>MSIQHFRVALIPFFAAFCLPVFAHPETLVKVKDAEDKLGARVGYIELDLNSGKILESFRPEERFPMMSTFKVLLCGAVLSRVDAGQEQLGRRIHYSQNDLVEYSPVTEKHLTDGMTVRELCSAAITMSDNTAANLLLTTIGGPKELTAFLHNMGDHVTRLDRWEPELNEAIPNDERDTTTPAAMATTLRKLLTGELLTL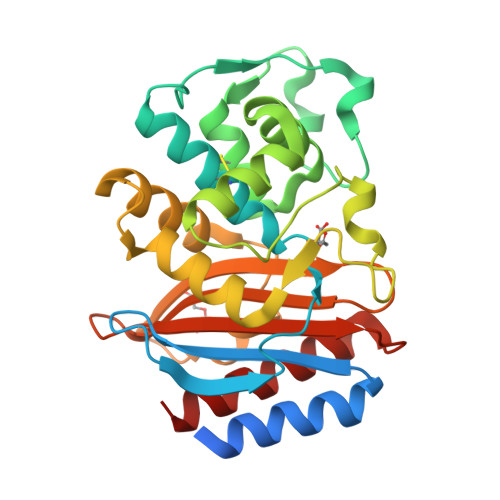ASRQQLIDWMEADKVAGPLLRSALPAGWFIADKSGASKRGSRGIIAALGPDGKPSRIVVIYTTGSQATMDERNRQIAEIGASLIKHW[2x]>MGSSHHHHHHSQMVSVIKPEMKIKLCMRGTVNGHNFVIEGEGKGNPYEGTQILDLNVTEGAPLPFAYDILTTVFQYGNRAFTKYPADIQDYFKQTFPEGYHWERSMTYEDQGICTATSNISMRGDCFFYDITFTGTNFPPNGPVMQKKTLKWEPSTEKMYVRDGVLKGDVNMALLLEGGGHYRCDFKT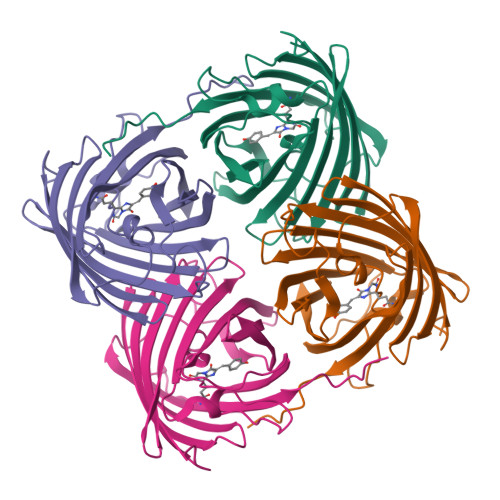TYKAKKDVRLPDYHFVDHRIEILKHDKDYNKVKLYENAVARYSMLPSQAK[4x]> MSDKLPTADSLRSMISGLGDPLRDKNASTFHWDRQLDDRQLLYAYRNSWVARKAVTIPALDAVRKWRDWQADQKDISRIEATEKRLGLQQKLLQCKTLARLWGGAAIVIGVKDQDMATPFEPETVNKDDLVYLTVMSRRELSPEELEQDPLDEFYARPKRYQVSNGRNLSFVHPSRIVHQVGETHPDPMLATGVNVGWGDSTLQALYDAMMNSDNTQANIASLVFEANVDVIGLPDFMENMSSEVYRQKLLDRFTLAAAGKGIN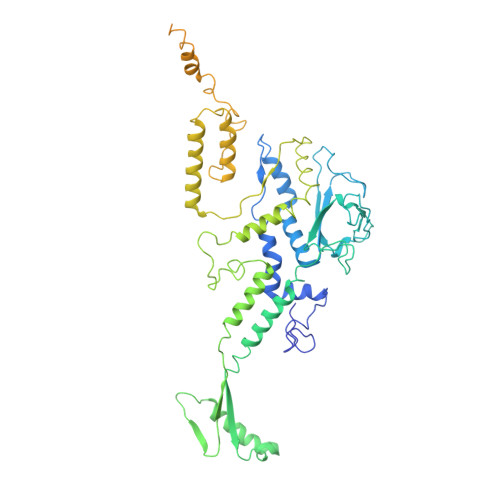KTLMLDAEEVFTAHSRSFANLDKIMEQFILFVAGAADIPLTRFLGQSPAGMSSTGQHDMKNYHDRIQSIQTLDLQPSMYRLDEAIIRSSLGARPEELFYIWSPLEQMSEKERAEIGKLHAETVNVIAGTGLFMQEELREVFGNQLVETGLYPGLGDLLAQNGNELPEWDLEQRSAEASTKTAEAAALAAETASRQPARAVTDATPRPLYMRRDVVNGDEILRHYREQGVEGLYAAEELHVTIAYSKKPLDWMKLGEPWSAKLEVAPGGPRVHELFGDDSSVLVLCFAASELNWRAQQVIDAGGSSDHGEYQSHISLSLQGRPEQIETLRPYQGRIVLGPELFEQIEEGDWREKVKTD1-(4-tert-butylphenyl)-2-[(1S,2R,5R,8R,8aR)-1,2,8-trihydroxyoctahydroindolizin-5-yl]ethanone 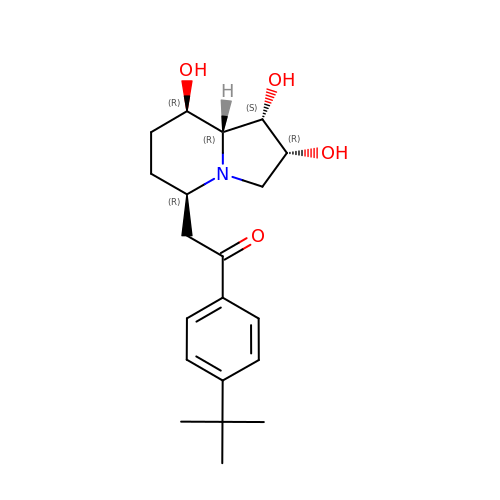| C20 H29 N O4 | PKZGDTMZYSPKOW-POGZOPGASA-N> MMQQRQVLMVEDTASVAALYKSYLNPLGLNVSIVGTGKEALSFIQDIIPDLILLDLRLPDMTGMEVLERVRKEHGNVPVVIMTAHGSIDIAVEAIRYGAQDFLIKPCEADRLRITVNKALKAESKSNTSTQSKQSDGAQYQGFIGNSLPMQAVYRVIESAASSKATVFITGESGTGKEVCAEAIHAASPRHDKPFIALNCAAIPKDLIESELFGHVKGAFTGASTERQGAVEMAHNGTLMLDELCEMDLDLQSKLLRFIQTGTYQKVGSSKMSSVDVRFVCATNRNPWEEVQEGRFREDLYYR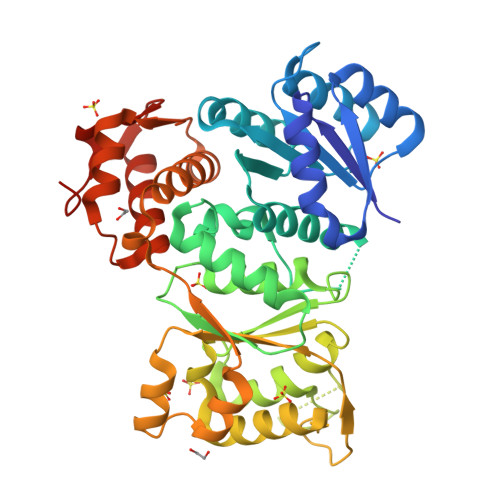LHVIPISLPPLRERGGDIIEIAHALLGLMSLEEGKSFSRFSEPVLRLFESYSWPGNVRELQNVIRNIVVLNTDDEVKLEMVPPPILEHHHHHH> GVYYATAYWMPTEKTIQVKNVLDRKGDAYGFYNNSVKTTGWGILEIKAGYGSQSLSNEIIMFAAGFLEGYLTAPHMDDHFTNLYPQLIKKRSMLNKVQDFLTKQDQWTRENIKYYKSDPFWRHADYVMAQMDGLFAGAT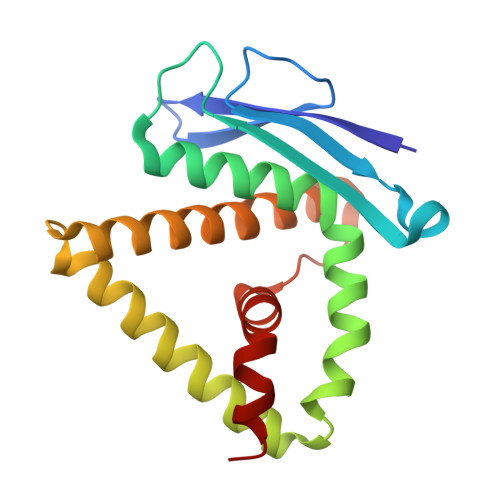KRAVLEGKKPMTLFQIQFLNAIGDLLDLIPS4-(4-{1-[(R)-amino(hydroxy)methyl-lambda~4~-sulfanyl]cyclopropyl}-6-[(3R)-3-methylmorpholin-4-yl]pyrimidin-2-yl)-1H-pyrrolo[2,3-b]pyridine | C20 H26 N6 O2 S | 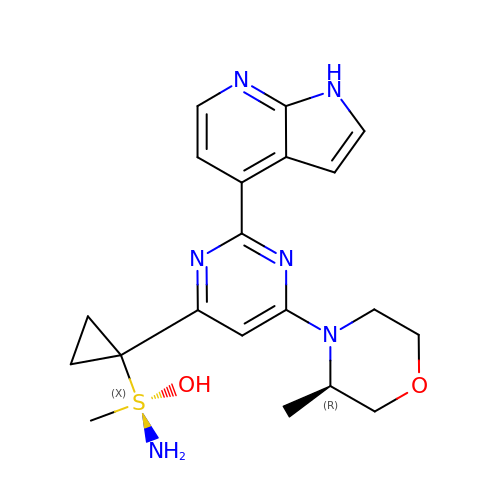UUSXGRTVICHEJW-CYBMUJFWSA-N>[2x]MRTHDDTWDIKTSVGTTAVMVAAARAAETDRPDALIRDPYAKLLVTNTGAGALWEAMLDPSMVAKVEAIDAEAAAMVEHMRSYQAVRTNFFDTYFNNAVIDGIRQFVILASGLDSRAYRLDWPTGTTVYEIDQPKVLAYKSTTLAEHGVTPTADRREVPIDLRQDWPPALRSAGFDPSARTAWLAEGLLMYLPATAQDGLFT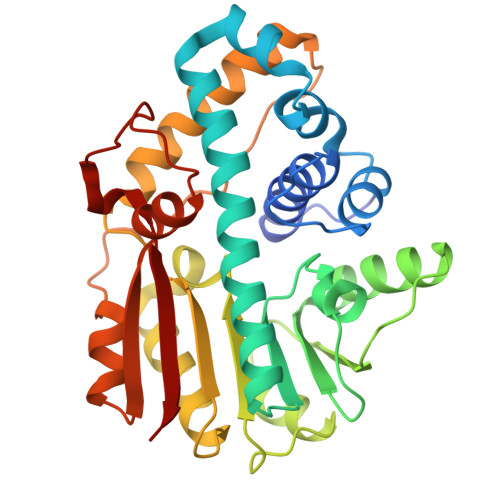EIGGLSAVGSRIAVETSPLHGDEWREQMQLRFRRVSDALGFEQAVDVQELIYHDENRAVVADWLNRHGWRATAQSAPDEMRRVGRWGDGVPMADDKDAFAEFVTAHRL>GGSIDETRAHLLLKEKMMRLGGRLVLNTKEELANERLMTLKIAEMKEAMRTLIFPPSMHFFQAKHLIERSQVFNILRMMPKGAALHLHDIGIVTMDWLVRNVTYRPHCHICFTPRGIMQFRFAHPTPRPSEKCSKWILLEDYRKRVQNVTEFDDSL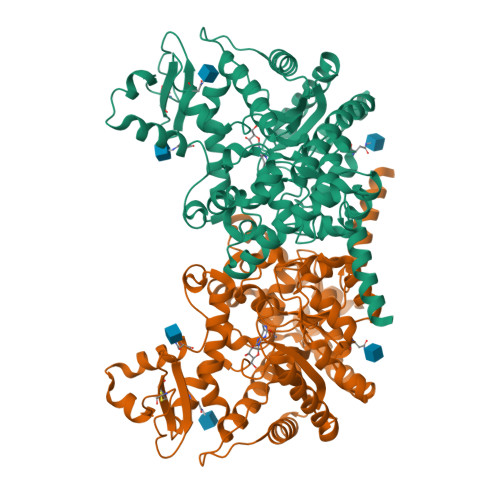LRNFTLVTQHPEVIYTNQNVVWSKFETIFFTISGLIHYAPVFRDYVFRSMQEFYEDNVLYMEIRARLLPVYELSGEHHDEEWSVKTYQEVAQKFVETHPEFIGIKIIYSDHRSKDVAVIAESIRMAMGLRIKFPTVVAGFDLVGHEDTGHSLHDYKEALMIPAKDGVKLPYFFHAGETDWQGTSIDRNILDALMLNTTRIGHGFALSKHPAVRTYSWKKDIPIEVCPISNQVLKLVSDLRNHPVATLMATGHPMVISSDDPAMFGAKGLSYDFYEVFMGIGGMKADLRTLKQLAMNSIKYSTLLESEKNTFMEIWKKRWDKFIADVATKGSLHHILDAQKMVWNHRHHHHHH[2x]>[2x]MSKEYHIDEEVGFALPNPQENLPDFYNDWMFIAKHLPDLIESGQLRERVEKLNMLSIDHLTDHKSQRLARLVLGCITMAYVWGKGHGDVRKVLPRNIAVPYCQLSKKLELPPILVYADCVLANWKKKDPNKPLTYENMDVLFSFRDGDCSKGFFLVSLLVEIAAASAIKVIPTVFKAMQMQERDTLLKALLEIASCLEKALQVFHQIHDHVNPKAFFSVLRIYLSGWKGNPQLSDGLVYEGFWEDPKEFAGGSAGQSSVGQCFDVLLGIQQTAGGGHAAQFLQDMRRYMPPAHRNFLCSLESNPSVREFVLSKGDAGLREAYDACVKALVSLRSYHLQIVTKYILIPASQQPKENKTSEDPSKLEAKGTGGTDLMNFLKTVRSTTEKSLLKEGKGELNSKLEGKPIPNPLLGLDSTRTGHHHHHH

hIDO1 is a heme-containing enzyme that catalyzes the first and rate-limiting step of the kynurenine pathway—the dioxygenation of Trp to N-formyl kynurenine (NFK). It negatively regulates cellular immune response via depleting Trp and promoting the accumulation of kynurenine pathway metabolites. HIDO1 is an α-helical protein, made up by a large C-terminal domain containing the Sa site and a small N-terminal domain sitting on top of it. Here we report the structures of the wild-type hIDO1 in complex with Trp, an inhibitor (epacadostat), and/or an effector (IDE), as well as comparable structures of an active site mutant, F270G.

We next crystallized the F270G-CN-Trp complex in the presence and absence of IDE, and solved their structures at a resolution of 2.69 and 3.03 Å, respectively. Remarkably, in the absence of IDE, electron density associated with Trp is evident in the Si site. It demonstrates that the Si site can indeed accommodate a second Trp, offering molecular explanation for the substrate inhibition behavior of the enzyme. The F270G data show that the Trp bound in the Si site adopts a unique conformation with respect to IDE. Specifically, its indole group flips 180°, such that the ammonium and carboxylate groups point away from the proprionate-6 group of the heme. The carboxylate and ammonium groups are in position to H-bond with E171/S267/G270 and V170, respectively, although their relatively weak density indicates that these potential H-bonding interactions are not strong. The E171 is fully conserved in IDO1 family of enzymes. In addition, it is only one helical turn away from S167 in the B-Helix, which directly interacts with the Trp bound in the Sa site, suggesting that it is a structural element mediating the structural communication between the Si and Sa sites. Although both the IDE complex and the two Trp-bound complex of the F270G mutant exhibit impeded enzyme activity, their structures are surprisingly similar to that of the wild-type complex, except that the heme is more planar and that the protein matrix is more flexible, in particular in the regions near the JK-LoopC, the K-Helix and D-Helix, as exemplified by the ability of the R231 sidechain to adopt two conformations in the IDE complex.> DLRPEIRIAQELRRIGDEFNETYTRRV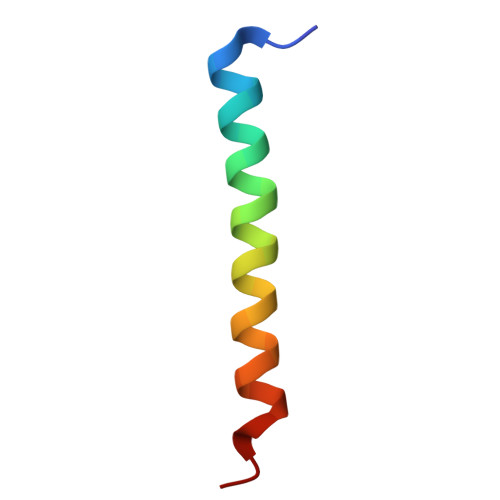FANDYR> AHKFAAPPCPNLLLLRKTIHQRLQPILFFLKNDVTMGNYVYDQ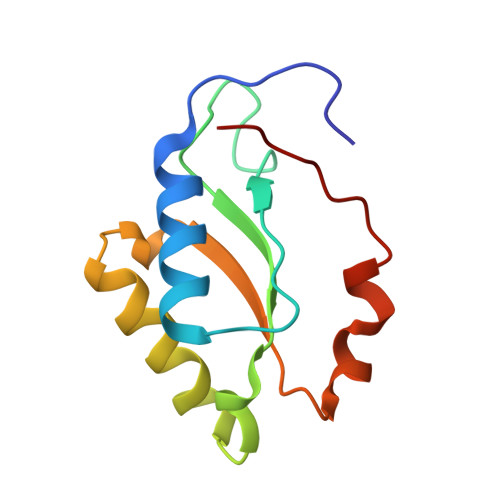HFKGVLCSPLFEGKSYKEIYAMVDRVLEDIGLSGRVKLYCEPPSLLHKMKYHVRKHWPLEKG> TDKNQTTQNNSSSPLTQVNTTVSVQIGTKALLCCFSIPLTKAVLITWIIKLRGLPSCTIAYKVDTKTNETSCLGRNITWASTPDHSPELQISAVTLQHEGTYTCETVTPEGNFEKNYDLQVLVPPEVTYFPEKNRSAVCEAMAGKPAAQISWSPDGDCVTTSESHSNGTVTVRSTCHWEQNNVSDVSCIVSHLTGNQSLSIELGRGGSTRHHHHHH;> QVEVVTQDERKALHTTASLRCSLKTSQEPLIVTWQKKKAVSPENMVTYSKTHGVVIQPAYKDRINVTELGLWNSSITFWNTTLEDEGCYMCLFNTFGSQKVSGTACLTLYVQPIVHLHYNYFEDHLNITCSATARPAPAISWKGTGTGIENSTESHFHSNGTTSVTSILRVKDPKTQVGKEVICQVLYLGNVIDYKQSLDKGSTRHHHHHH

CD200 is a widely distributed membrane glycoprotein that regulates myeloid cell activity through its interaction with an inhibitory receptor (CD200R). CD200R is a member of a “paired receptor” family as in addition to this inhibitory receptor there is one very closely related gene with activating potential in humans and several in mice (Akkaya and Barclay, 2010; Wright et al., 2003). We report X-ray crystallography structures for the inhibitory CD200R, the activating receptor CD200RLa, and a complex between CD200R and CD200.

The coordinates of CD200R were used as a MR search model for the CD200R/CD200 complex and CD200 was built in a map calculated using partial MR phases. The structure of CD200 was solved in complex with CD200R and contains an NH2-terminal Ig V-like domain followed by a smaller C2-like domain. The structure of the CD200/CD200R complex shows near orthogonal binding of the V-like domains of each molecule, whereby the CD200 FCC′C″ face and CC′ and FG loops form a concave surface that embraces the relatively flat AGFCC′C″ face and FG loop of CD200R. The CD200/CD200R interaction buries a total of 1768 Å2 of solvent-accessible area (901 Å2 from CD200 and 868 Å2 from CD200R) and shows high shape complementarity with a shape correlation score (SC) of 0.69. The interaction interface also shows charge complementarity with acidic patches on CD200R complementing basic patches on CD200 where a network of polar interactions is clustered. There are two salt bridges with K100 (FG loop) of CD200-forming salt bridges with E106 (beta strand F) and E115 (beta strand G) of CD200R. In particular F96 (in the FG loop) of CD200 mediates numerous hydrophobic interactions where the phenyl ring sits in a hydrophobic pocket formed by residues in the CD200R CC′C″ beta sheet (L45, A61, Y62, K63, T68, N69, and E70). Despite the high content of carbohydrate in both CD200 and CD200R, it is not involved in the interaction, with N-linked glycosylation of both CD200 and CD200R distant from the interface with the exception of N20 of CD200R, which lies at the periphery of the interaction interface. In addition to a disulfide bond between beta strands B and F in both IgSF domains of CD200, there is an exposed disulfide bond between beta strands F and G in the V-like domain. The distance between the last residues of each molecule in the structural model is ∼12 nm; this appears somewhat smaller than the 14 nm typically found for protein interactions spanning the immunological synapse; however, a further nine residues of CD200R need to be accounted for before entering the predicted transmembrane region.>MGHHHHHHSHMADNMTTTQIEVGPGATNATINFEAGILECYERFSWQRALDYPGQDRLHRLKRKLESRIKTHNKSEPENKRMSLEERKAIGVKMMKVLLFMDPSAGIEGFEPY[2x];>[2x]SHHHHHHMGWDLTVKMLAGNEFQVSLSSSMSVSELKAQITQKIGVHAFQQRLAVHPSGVALQDRVPLASQGLGPGSTVLLVVDKCDEPLSILVRNNKGRSSTYEVRLTQTVAHLKQQVSGLEGVQDDLFWLTFEGKPLEDQLPLGEYGLKPLSTVFM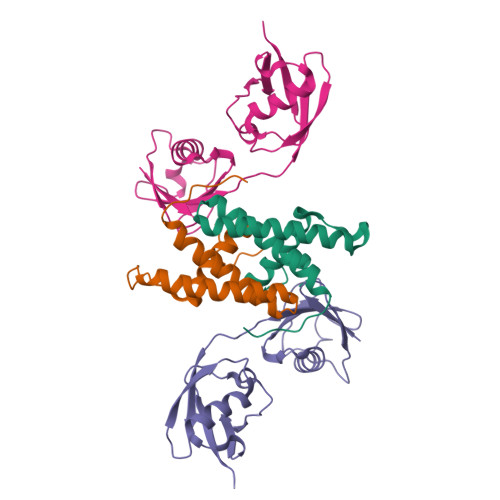NLRLRGG>MSLKQKRPKYMQIIDAAVEVIAENGYHQSQVSKIAKQAGVADGTIYLYFKNKEDILISLFKEKMGQFIERMEEDIKEKAT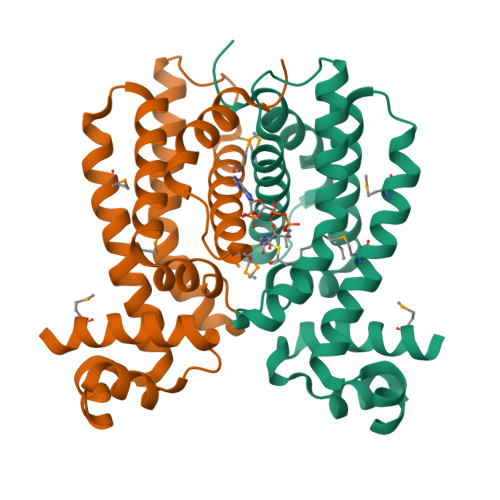AKEKLALVISKHFSLLAGDHNLAIVTQLELRQSNLELRQKINEILKGYLNILDGILTEGIQSGEIKEGLDVRLARQMIFGTIDETVTTWVMNDQKYDLVALSNSVLELLVSGIHNKEGGSHHHHHH[2x]> IENPQYFSDACVHHIKRRDIVLKWELGEGAFGKVFLAECHNLLPEQDKMLVAVKALKEASESARQDFQREAELLTMLQHQHIVRFFGVCTEGRPLLMVFEYMRHGDLNRFLRSH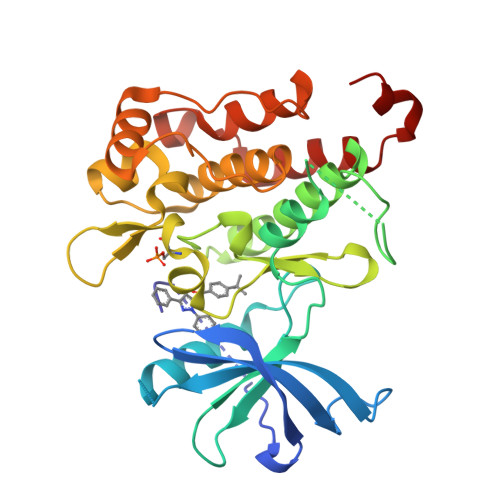GPDAKLLAGGEDVAPGPLGLGQLLAVASQVAAGMVYLAGLHFVHRDLATRNCLVGQGLVVKIGDFGMSRDIYSTDYYRVGGRTMLPIRWMPPESILYRKFTTESDVWSFGVVLWEIFTYGKQPWYQLSNTEAIDCITQGRELERPRACPPEVYAIMRGCWQREPQQRHSIKDVHARLQALAQAPPVYLDVL>[2x]MDLGEFPAPDPSVLVQNFNISDFNGKWYITSGLNPTFDAFDCQLHEFHTEGDNKLVGNISWRIKTLDSGFFTRSAVQKFVQDPNQPGVLYNHDNEYLHYQDDWYILSSKIE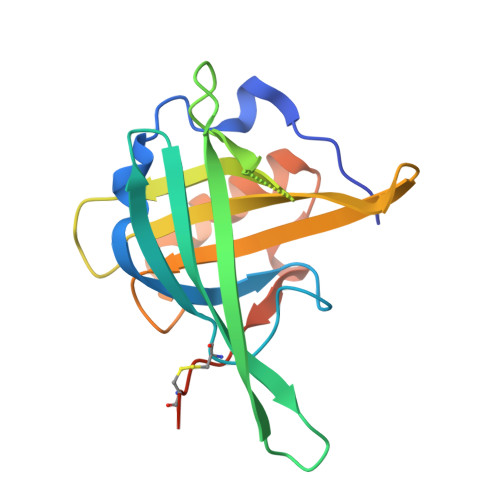NKPEDYIFVYYRGRNDAWDGYGGAVVYTRSSVLPNSIIPELEKAAKSIGRDFSTFIRTDNTCGPEPRSHHHHHH N-[4-chloro-3-(morpholin-4-yl)phenyl]-N~2~-[3-(hydroxymethyl)quinolin-6-yl]-L-alaninamide | C23 H25 Cl N4 O3 | 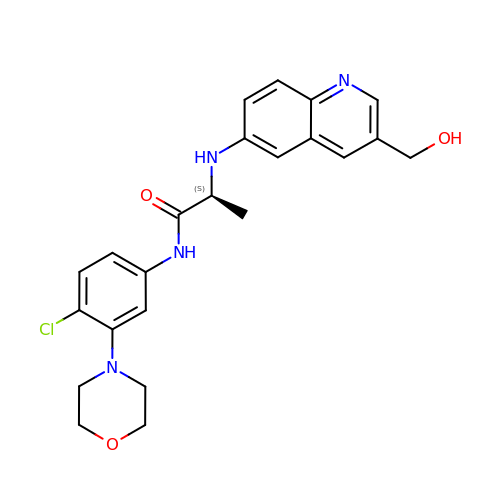VDBAUTDBXIRAKX-HNNXBMFYSA-N> MAKQYDSVECPFCDEVSKYEKLAKIGQGTFGEVFKARHRKTGQKVALKKVLMENEKEGFPITALREIKILQLLKHENVVNLIEICRTKASPYNRCKGSIYLVFDFCEHDLAGLLSNVLVKFTLSEIKRVMQMLLNGLYYIHRNKILHRDMKAANVLITRDGVLKLADFGLARAFSLAKNSQPNRYTNRVVTLWYRPPELLLGERDYGPPIDLWGAGCIMAEMWTRSPIMQGNTEQHQLALISQLCGSITPEVWPNVDNYELYEKLELVKGQKRKVKDRLKAYVRDPYALDLIDKLLVLDPAQRIDSDDALNHDFFWSDPMPSDLKGMLST;> EGERKNNNKRWYFTREQLENSPSRRFGVDPDKELSYRQQAANLLQDMGQRLNVSQLTINTAIVYMHRFYMIQSFTRFPGNSVAPAALFLAAKVEGQPKKLEHVIKVAHTCLHPQESLPDTRSEAYLQQVQDLVILESIILQTLGF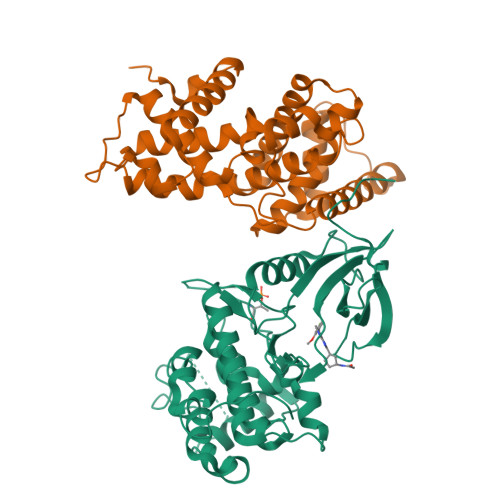ELTIDHPHTHVVKCTQLVRASKDLAQTSYFMATNSLHLTTFSLQYTPPVVACVCIHLACKWSNWEIPVSTDGKHWWEYVDATVTLELLDELTHELLQILEKTPNRLKRIWNWR> MEHEKDPGWQYLRRTREQVLEDQSKPYDSKKNVWIPDPEEGYLAGEITATKGDQVTIVTARGNEVTLKKELVQEMNPPKFEKTEDMSNLSFLNDASVLHNLRSRYAAMLIYTYSGLFCVVINPYKRLPIYTDSCARMFMGKRKTEMPPHLFAVSDEAYRNMLQDHENQSMLITGESGAGKTENTKKVICYFAAVGASQQEGGAEVDPNKKKVTLEDQIVQTNPVLEAFGNAKTVRNNNSSRFGKFIRIHFNKHGRLASCDIEHYLLEKSRVIRQAPGERCYHIFYQIYSDFRPELKKELLLDLPIKDYWFVAQAELIIDGIDDVEEFQLTDEAFDILNFSAVEKQDCYRLMSAHMHMGNMKFKQRPREEQAEPDGTDEAEKASNMYGIGCEEFLKALTKPRVKVGTEWVSKGQNCEQVNWAVGAMAKGLYSRVFNWLVKKCNLTLDQKGIDRDYFIGVLDIAGFEIFDFNSFEQLWINFVNEKLQQFFNHHMFVLEQEEYAREGIQWVFIDFGLDLQACIELIEKPLGIISMLDEECIVPKATDLTLASKLVDQHLGKHPNFEKPKPPKGKQGEAHFAMRHYAGTVRYNCLNWLEKNKDPLNDTVVSAMKQSKGNDLLVEIWQDYTTQEEAAAKAKEGGGGGKKKGKSGSFMTVSMLYRESLNNLMTMLNKTHPHFIRCIIPNEKKQSGMIDAALVLNQLTCNGVLEGI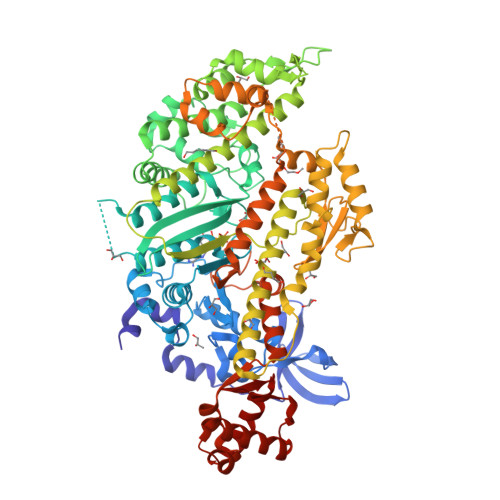RICRKGFPNRTLHPDFVQRYAILAAKEAKSDDDKKKCAEAIMSKLVNDGSLSEEMFRIGLTKVFFKAGVLAHLEDIRDEKL>[2x]QAQITGRPEWIWLALGTALMGLGTLYFLVKGMGVSDPDAKKFYAITTLVPAIAFTMYLSMLLGYGLTMVPFGGEQNPIYWARYADWLFTTPLLLLDLALLVDADQGTILALVGAAGIMIG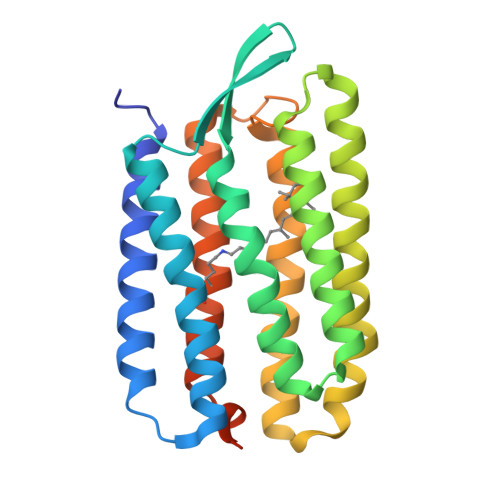TGLVGALTKVYSYRFVWWAISTAAMLYILYVLFFGFTSKAESMRPEVASTFKVLRNVTVVLWSAYPVVWLIGSEGAGIVPLNIETLLFMVLDVSAKVGFGLILLRSRAIFGEAEAPEPSAGDGAAATSD>GPGSMVTIAEIAGRTLTQERRLVTAIPGPISQELQARKQSAVAAGVGVTLPVYVVAAGGGVLADADGNQLIDFGSGIAVTTVGNSAPAVVDAVTQQVAAFTHTCFMVTPYEGYVKVAEHLNRLTPGDHEKRTALFNSGAEAVENAVKIARAYTRRQAVVVFDHAYHGRTNLTMAMTAKNQPYKHGFGPFANEVYRVPTSYPFRDGETDGAAAAAHALDLINKQVGADNVAAVVIEPVHGEGGFVVPAPGFLGALQKWCTDNGAVFVADEVQTGFARTGALFACEHENVVPDLIVTAKGIAGGLPLSAVTGRAEIMDGPQSGGLGGTYGGNPLACAAALAVIDTIERENLVARARA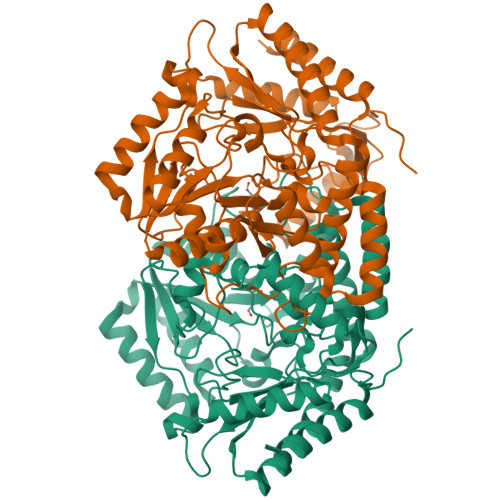IGETMLSRLGALAAADPRIGEVRGRGAMIAVELVKPGTTEPDADLTKRVAAAAHAQGLVVLTCGTYGNVLRFLPPLSMPDHLLDEGLDILAAVFAEVK[4x]>MPLNPHVEALLQMMAQMPAPDFSVANPAEIRAVFDNLAAPPQVARVENIAISLDGRDLDARLYVPEDADERPALMVYYHGGGWVIGTLDTHDGTCRALAQKSGCAVLSIAYRLAPEYRYPAPAEDCYDALVWAKQNAATLGVDGDRLAVGGDAAGGNLAAAVAIMARDRNGPALRHQLLIYPVTDNDFTLA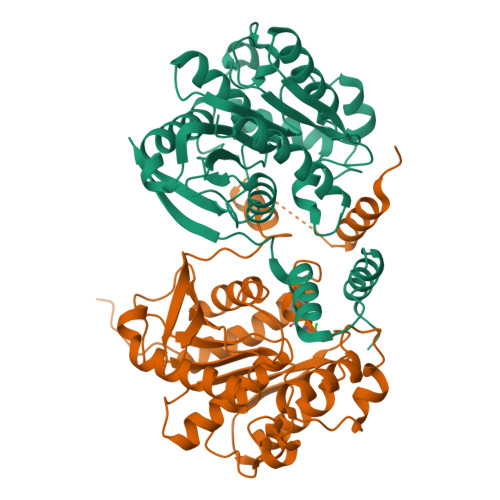SYAENGGGEYYLSTDGMRWFWGHYLGDTAAENAPLAAVLNVADLSGLAPATVITAEYDPLRDEGIAYAKKLDAAGVPVDAATAPGMIHGFFSMFEAVPDSWEWIERGASNLKRDLALEHHHHHHHH[2x]>[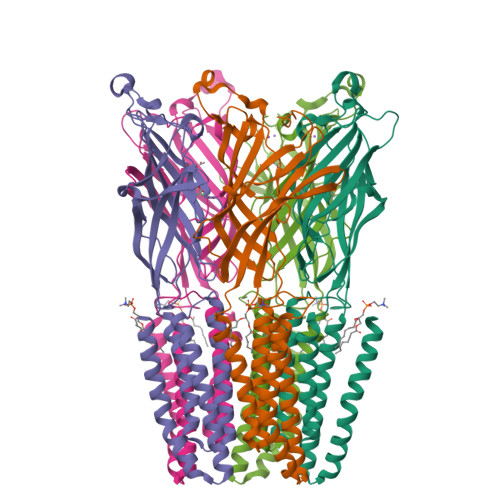5x]AQDMVSPPPPIADEPLTVNTGIYLIECYSLDDKAETFKVNAFLSLSWKDRRLAFDPVRSGVRVKTYEPEAIWIPEIRFVNVENARDADVVDISVSPDGTVQYLERFSARVLSPLDFRRYPFDSQTLHIYLIVRSVDTRNIVLAVDLEKVGKNDDVFLTGWDIESFTAVVKPANFALEDRLESKLDYQLRISRQYFSYIPNIILPMLFILFISWTAFWSTSYEANVTLVVSTLIAHIAANILVETNLPKTPYMTYTGAIIFMIYLFYFVAVIEVTVQHYLKVESQPARAASITRASRIAFPVVFLLANIILAFLFFGF> MASFIDLFAGDITTQLLKLLALVANTVYSCKGIAERLITMIRDVQPTIREIQYSGAELSNHHQTQLGVFYEILEKARKLCEKVLRCNRWNLKHVYHANKMKDLEKQISRFLNSQILLFVLAEVCHLRVNGDRIERNMDRLLTERNDSLSFPETMMEIETVSDPEIQTVLELGKKKVKEMMFKFTDTHLFGISGMSGSGKTTLAIELSKDDDVR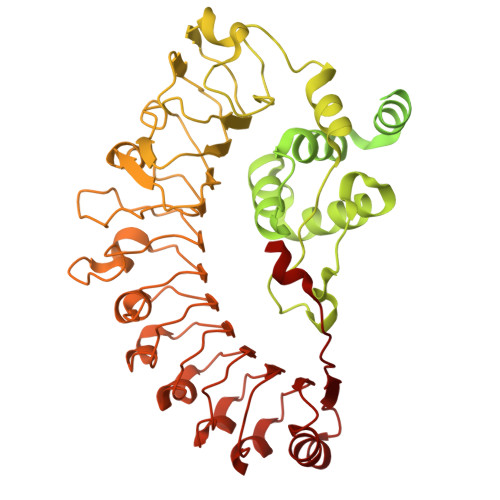GLFKNKVLFLTVSRSPNFENLESCIREFLYDGVHQRKLVILDDVWTRESLDRLMSKIRGSTTLVVSRSKLADPRTTYNVELLKKDEAMSLLCLCAFEQKSPPSPFNKYLVKQVVDECKGLPLSLKVLGASLKNKPERYWEGVVKRLLRGEAADETHESRVFAHMEESLENLDPKIRDCFLDMGAFPEDKKIPLDLLTSVWVERHDIDEETAFSFVLRLADKNLLTIVNNPRFGDVHIGYYDVFVTQHDVLRDLALHMSNRVDVNRRERLLMPKTEPVLPREWEKNKDEPFDAKIVSLHTGEMDEMNWFDMDLPKAEVLILNFSSDNYVLPPFIGKMSRLRVLVIINNGMSPARLHGFSIFANLAKLRSLWLKRVHVPELTSCTIPLKNLHKIHLIFCKVKNSFVQTSFDISKIFPSLSDLTIDHCDDLLELKSIFGITSLNSLSITNCPRILELPKNLSNVQSLERLRLYACPELISLPVEVCELPCLKYVDISQCVSLVSLPEKFGKLGSLEKIDMRECSLLGLPSSVAALVSLRHVICDEETSSMWEMVKKVVPELCIEVAKKCFTVDWLDD> 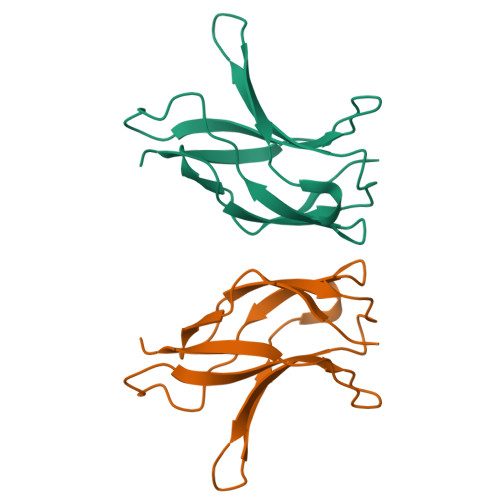ASNLKIVRMDRTAGCVTGGEEIMLLCDKVQKDDIQIRFYEEEENGGVWEGFGDFSPTDVHRQFAICFKTPKYKDVNITKPASVFVQLRRKSDLETSEPKPFLYYPE> VANPEHYIKHPLQNRWALWFFKNDKSKTWQANLRLISKFDTVEDFWALYNHIQLSSNLMPGCDYSLFKDGIEPMWEDEKNKRGGRWLITLNKQQRRSDLDRFWLETLLCLIGESFDDYSD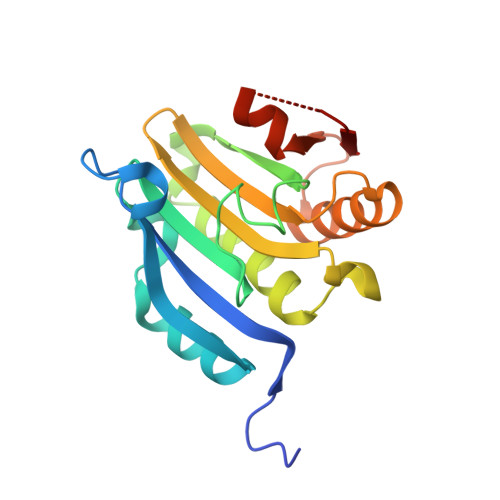DVCGAVVNVRAKGDKIAIWTTECENRDAVTHIGRVYKERLGLPPKIVIGYQSHADTATKSGSTTKNRFVV PLK4, and this interaction targets STIL to centrioles. allows homo-multimerisation, the interaction with the PB3 domain of PLK4, or both. structures and interactions of CCDs and PLK4-PB3s in humans and flies. STIL/Ana2, which can then interact with and recruit Sas-6.

structure of the strand swapped dimers is unambiguous. similar to that seen in the mouse PB3 crystal (MmPB3, grey cartoon). mouse PB3 domain behaving as an unusual strand-swapped dimer. crystal structures of the human (this study) and mouse PB3. monomer, with the multimeric forms dominating.

>[60x]GPMGSAQLLKSVFVKNVGWATQLTSGAVWVQFNDGSQLVVQAGVSSISYTSPNGQTTRYGENEKLPDYIKQKLQCLSSILLMFSNPTPNFH> ALINPQFPYAGPVPIPGPAPTETMPLLNYRVEGRIAGIQQARQFMPFL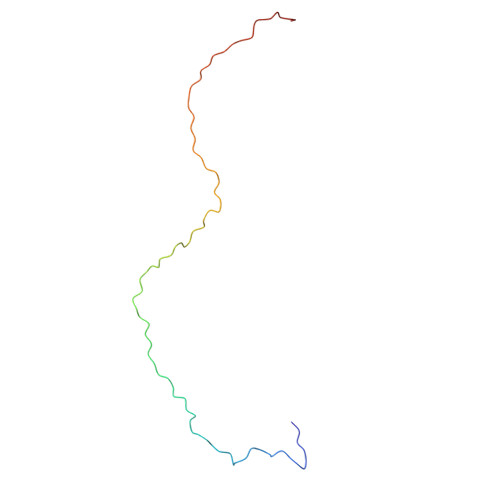QGPHRAVAEQTYHAIGTGIQMGQTFNQPLINTQEG> MTLEKFVDALPIPDTLKPVQQSKEKTYYEVTMEECTHQLHRDLPPTRLWGYNGLFPGPTIEVKRNENVYVKWMNNLPSTHFLPIDHTIHHSDSQHEEPEVKTVVHLHGGVTPDD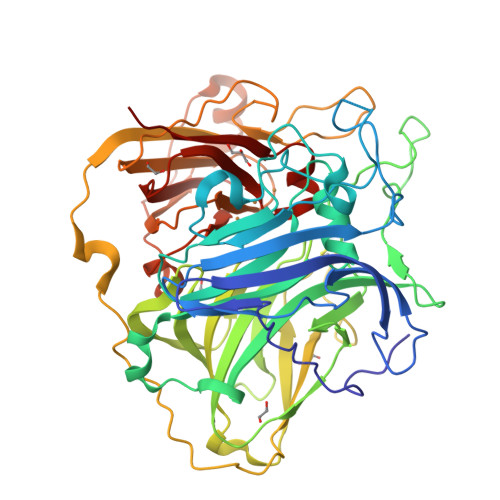SDGYPEAWFSKDFEQTGPYFKREVYHYPNQQRGAILWYHDHAMALTRLNVYAGLVGAYIIHDPKEKRLKLPSDEYDVPLLITDRTINEDGSLFYPSAPENPSPSLPNPSIVPAFCGETILVNGKVWPYLEVEPRKYRFRVINASNTRTYNLSLDNGGDFIQIGSDGGLLPRSVKLNSFSLAPAERYDIIIDFTAYEGESIILANSAGCGGDVNPETDANIMQFRVTKPLAQKDESRKPKYLASYPSVQHERIQNIRTLKLAGTQDEYGRPVLLLNNKRWHDPVTETPKVGTTEIWSIINPTRGTHPIHLHLVSFRVLDRRPFDIARYQESGELSYTGPAVPPPPSEKGWKDTIQAHAGEVLRIAATFGPYSGRYVWHCAILEHEDYDMMRPMDITDPHK(3~{R})-piperidin-3-ol 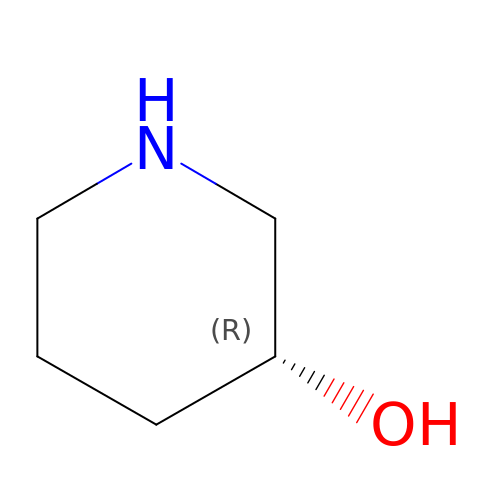| C5 H11 N O | BIWOSRSKDCZIFM-RXMQYKEDSA-N>AHRDSGTAKSGLYVEKVSGLRKDFIKGVDVSSIIALEESGVAFYNESGKKQDIFKTLKEAGVNYVRVRIWNDPYDANGNGYGGGNNDLEKAIQIGKRATANGMKLLADFHYSDFWADPAKQKAPKAWANLNFEDKKTALYQYTKQSLKAMKAAGIDIGMVQVGNETNGGLAGETDWAKMSQLFNAGSQAVRETDSNILVALHFTNPETSGRYAWIAETLHRHHVDYDVFASSYYPFWHGTLKNLTSVLTSVADTYGKKVM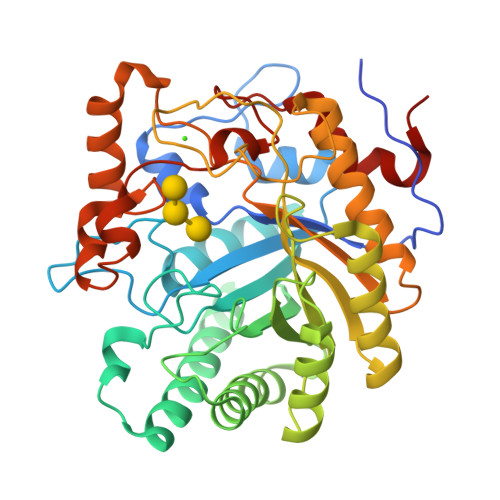VAATSYTYTAEDGDGHGNTAPKNGQTLNNPVTVQGQANAVRDVIQAVSDVGEAGIGVFYWEPAWIPVGPAHRLEKNKALWETYGSGWATSYAAEYDPEDAGKWFGGSAVDNQALFDFKGRPLPSLHVFQYVDTGTPFKN[2x]> GSSMKASSGDQGSPP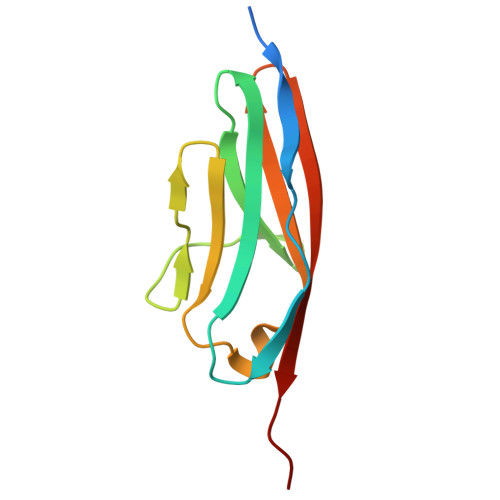CFLRRPRPVRVVSGAEAELKCVVLGEPPPVVVWEKGGQQLAASERLSFPADGAEHGLLLTAALPTDAGVYVCRARNAAGEAYAAAAVTVLEPPA> GSFTMDHYLDIRLRPDPEFPPAQLMSVLFGKLHQALVAQGGDRIGVSFPDLDESRSRLGERLRIHASADDLRALLARPW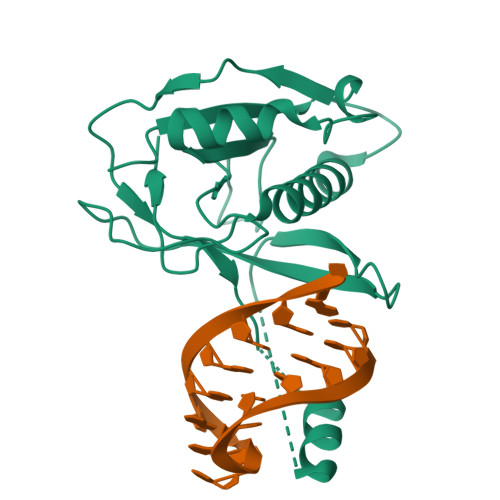LEGLRDHLQFGEPAVVPHPTPYRQVSRVQAKSNPERLRRRLMRRHDLSEEEARKRIPDTVARTLDLPFVTLRSQSTGQHFRLFIRHGPLQVTAEEGGFTCYGLSKGGFVPWF>MTQQPFQLPHFYLPHPARLNPHLDEARAHSTTWAREMGMLEGSGVWEQSDLEAHDYGLLCAYTHPDCDGPALSLITDWYVWVFFFDDHFLEKYKRSQDRLAGKAHLDRLPLFMPLDDAAGMPEPRNPVEAGLADLWTRTVPAMSADWRRRFAVATEHLLNESM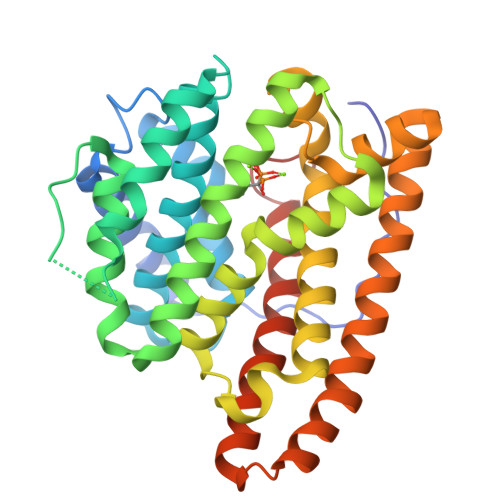WELSNINEGRVANPVEYIEMRRKVGGAPWSAGLVEYATAEVPAAVAGTRPLRVLMETFSDAVHLRNDLFSYQREVEDEGELSNGVLVLETFFGCTTQEAADLVNDVLTSRLHQFEHTAFTEVPAVALEKGLTPLEVAAVGAYTKGLQDWQSGGHEWHMRSSRYMNKGERPLAGWQ[2x]4-[2-[(2~{R})-2-[3-propyl-6-(trifluoromethyloxy)-1~{H}-indol-2-yl]piperidin-1-yl]ethyl]morpholine | C23 H32 F3 N3 O2 | 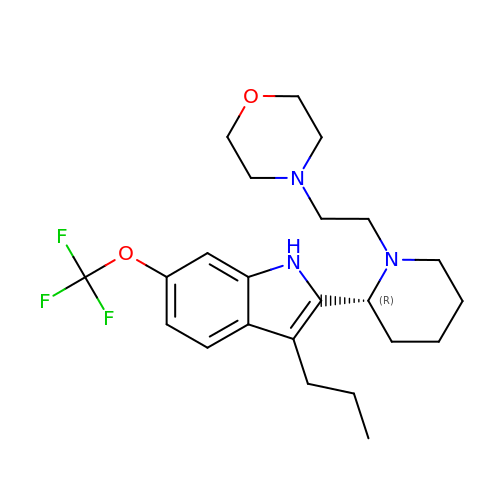UNPIVXUWRQMOQC-OAQYLSRUSA-N> GSMEYEWKPDEQGLQQILQLLKESQSPDTTIQRTVQQKLEQLNQYPDFNNYLIFVLTKLKSEDEPTRSLSGLILKNNVKAHFQNFPNGVTDFIKSECLNNIGDSSPLIRATVGILITTIASKGELQNWPDLLPKLCSLLDSEDYNTCEGAFGALQKICEDSAEILDSDVLDRPLNIMIPKFLQFFKHSSPKIRSHAVACVNQFIISRTQALMLHIDSFIENLFALAGDEEPEVRKNVCRALVMLLEVRMDRLLPHMHNIVEYMLQRTQDQDENVALEACEFWLTLAEQPICKDVLVRHLPKLIPVLVNGMKYSDIDIILLKGDVEEDETIPDSEQDIRGGSGGSGDTISDWNLRKCSAAALDVLANVYRDELLPHILPLLKELLFHHEWVVKESGILVLGAIAEGCMQGMIPYLPELIPHLIQCLSDKKALVRSITCWTLSRYAHWVVSQPPDTYLKPLMTELLKRILDSNKRVQEAACSAFATLEEEACTELVPYLAYILDTLVFAFSKYQHKNLLILYDAIGTLADSVGHHLNKPEYIQMLMPPLIQKWNMLKDEDKDLFPLLECLSSVATALQSGFLPYCEPVYQRCVNLVQKTLAQAMLNNAQPDQYEAPDKDFMIVALDLLSGLAEGLGGNIEQLVARSNILTLMYQCMQDKMPEVRQSSFALLGDLTKACFQHVKPCIADFMPILGTNLNPEFISVCNNATWAIGEISIQMGIEMQPYIPMVLHQLVEIINRPNTPKTLLENTAITIGRLGYVCPQEVAPMLQQFIRPWCTSLRNIRDNEEKDSAFRGICTMISVNPSGVIQDFIFFCDAVASWINPKDDLRDMFCKILHGFKNQVGDENWRRFSDQFPLPLKERLAAFYGV;> GGSRGGYDRGGYRGRGGDRGGFRGGRGGGDRGGFGPGKMDSRGEHRQDRRERLY

The nuclear import receptor Karyopherin β2 (Kapβ2, also known as Transportin-1 or TNPO1) imports FUS into the nucleus, where it functions in DNA repair, transcriptional regulation, mRNA and miRNA processing, and in RNA shuttling and stabilization. Kapβ2 imports WT FUS by binding tightly to the FUSPY-NLS (residues 501–526), with a dissociation constant (KD) of ~ 50 nM. However, mutations related to the PY-NLS of FUS (FUSPY-NLS) cause the FUS variants to localize to different extents to the cytoplasm and cause different degrees of disease severity in patients.

Although the FUSPY-NLS peptide carrying the P525L mutation binds Kapβ2 weaker than the WT FUSPY-NLS, it still binds Kapβ2 with substantial affinity (KD 180 nM), which allowed assembly of the Kapβ2·FUS(P525L)PY-NLS complex for structure determination by X-ray crystallography. We solved the crystal structure of the FUS(P525L)PY-NLS in complex with Kapβ2 (dissociation constant, KD = 180 nM) to 2.7 Å resolution, by molecular replacement. Residues 507–526 of the bound FUS(P525L)PY-NLS peptide were modeled. The FUS(P525L)PY-NLS-bound Kapβ2 is almost identical to WT FUSPY-NLS-bound Kapβ2 (root-mean square deviations or rmsd of 0.5 Å for 784 aligned Cα atoms). Epitope-1 (residues 508–511) and epitope-2 (residues 514–522) of FUS(P525L)PY-NLS bind Kapβ2 almost exactly the same as WT PY-NLS. Structural differences are observed only in epitope-3 (residues 525 and 526) where the ALS mutation resides. The P525L mutation changes the structure of the PY-NLS main chain from residues 522–525, which diverged from the peptide main chain of the WT PY-NLS and moved slightly farther away from Kapβ2. The L525 side chain of FUS(P525L)PY-NLS makes fewer contacts with Kapβ2 W460 and I457, and is too far away to interact with the L419 side chain of Kapβ2. There is no observed electron density for the E523 and R524 side chains of FUS(P525L)PY-NLS even though these side chains have well-defined electron density in the Kapβ2-bound WT FUSPY-NLS structure where E523 contacts the karyopherin and R524 participates in intra-peptide interactions. In summary, the P525L mutation caused local structural changes that resulted in fewer contacts with Kapβ2 and in the loss of potentially stabilizing intra-peptide interactions, all contributing to a significant loss of affinity for the importin.> MHHHHHHDDDDKRTLPGEGTQVHPRAPLLQILKVAGAQEEVFTVKEVMHYLGQY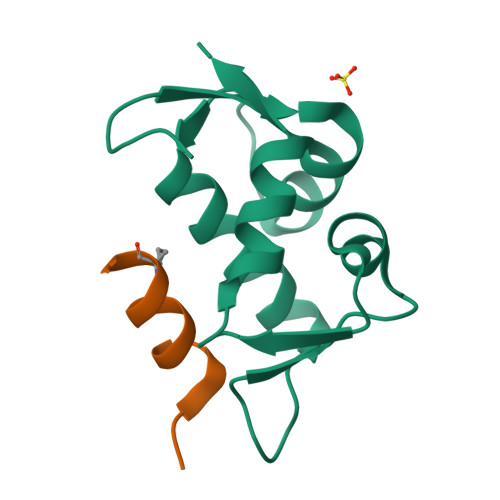IMMKQLYDKQRQHIVHCHDDPLGELLEVGSFSVKNPSPLYEMLKRNLVIL;> QSQQTFXNLWRLELQNX>GSKKHTGYVGLKNQGATCYMNSLLQTLFFTNQLRKAVYMMPTEGDDSSKSVPLALQRVFYELQHSDKPVGTKKLTKSFGWETLDSFMQHDVQELCRVLLDNVENKMKGTCVEGTIPKLFRGKMVSYIQCKEVDYRSDRREDYYDIQLSIKGKKNIFESFVDYVAVEQLDGDNKYDAGEHGLQEAEKGVKFLTLPPVLHLQLMRFMYDPQTDQNIKINDRFEFPEQL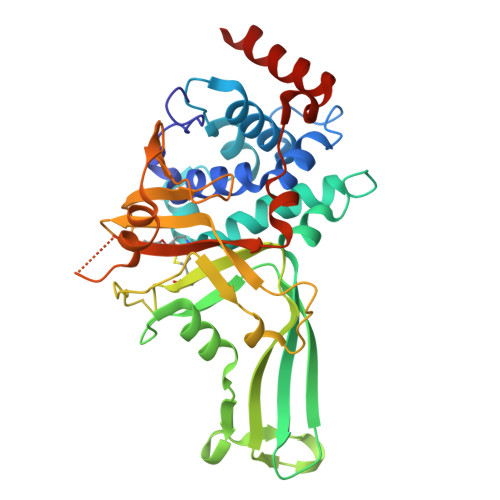PLDEFLQKTDPKDPANYILHAVLVHSGDNHGGHYVVYLNPKGDGKWCKFDDDVVSRCTKEEAIEHNYGGHDDDLSVRHCTNAYMLVYIRESKLSEVLQAVTDHDIPQQLVERLQEEKRIEAQKR[2x]>[2x]MSSIEWNEKTFAKF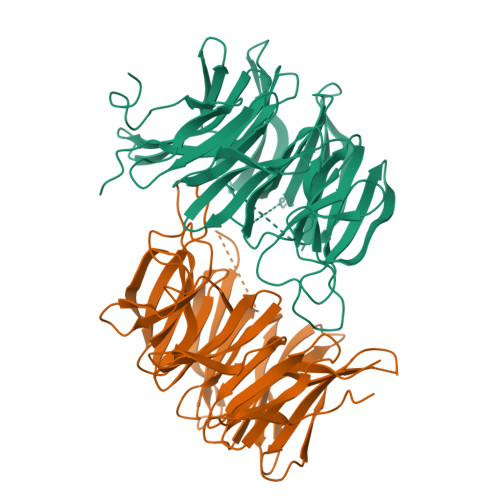AYLSDPRTKGELVAYVLTKANLKDNKYENTIVIENLKNNARRFIENATMPRISPDGKKIAFMRANEEKKVSEIWVADLETLSSKKILEAKNIRSLEWNEDSRKLLIVGFKRREDEDFIFEDDVPAWFDDLGFFDGEKTTFWIFDTESEEVIEEFEKPRFSSGIWHRDKIVVNVPHREIIPQYFKFWDIYIWEDGKEEKMFEKVSFYAVDSDGERILLYGKPEKKYMSEHNKLYIYDGKEVMGILDEVDRGVGQAKIKDGKVYFTLFEEGSVNLYIWDGEIKPIAKGRHWIMGFDVDEIVVYLKETATRLRELFTWDGEEKQLTDYNDPIFAKL>[2x]AKMKLYNFWRSGTSHRLRIALNLKG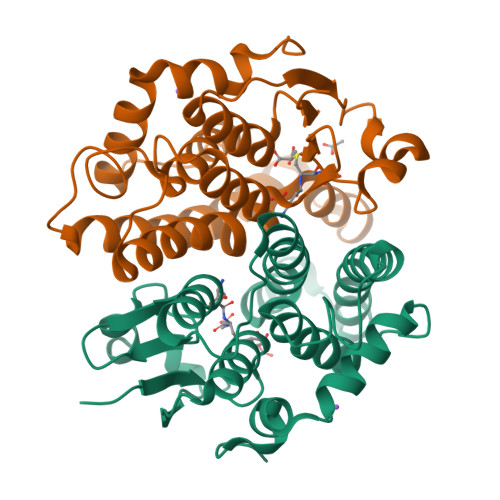VPYEYLAVHLGKEEHLKDAFKALNPQQLVPALDTGAQVLIQSPAIIEWLEEQYPTPALLPADADGRQRVRALAAIVGCDIHPINNRRILEYLRKTFGADEAAINAWCGTWISAGFDAYEALLAVDPKRGRYSFGDTPTLADCYLVPQVESARRFQVDLTPYPLIRAVDAACGELDAFRRAAPAAQPDSA> MAIYADNSYSIGNTPLVRLKHFGHNGNVVVKIEGRNPSYSVKCRIGANMVWQAEKDGTLTKGKEIVDATSGNTGI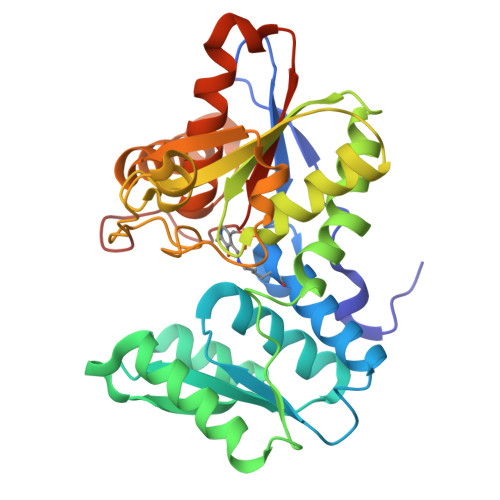ALAYVAAARGYKITLTMPETMSLERKRLLCGLGVNLVLTEGAKGMKGAIAKAEEIVASDPSRYVMLKQFENPANPQIHRETTGPEIWKDTDGKVDVVVAGVGTGGSITGISRAIKLDFGKQITSVAVEPVESPVISQTLAGEEVKPGPHKIQGIGAGFIPKNLDLSIIDRVETVDSDTALATARRLMAEEGILAGISSGAAVAAADRLAKLPEFADKLIVVILPSASERYLSTALFEGIEG>MGRVRLVQFQKNTDEPMGITLKMNELNHCIVA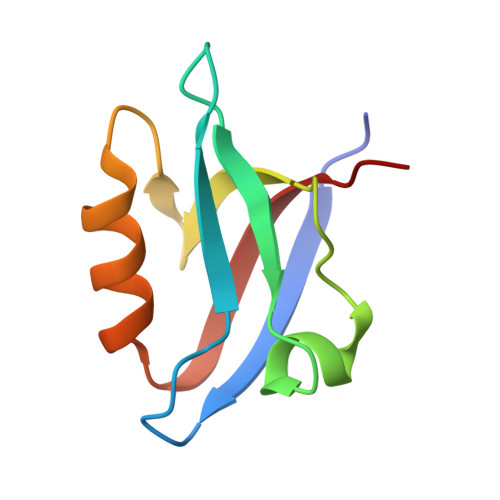RIMHGGMIHRQGTLHVGDEIREINGISVANQTVEQLQKMLREMRGSITFKIVPSYR[3x]>PRSLANAPIMILNGPNLNLLGQRQPEIYGSDTLADVEALCVK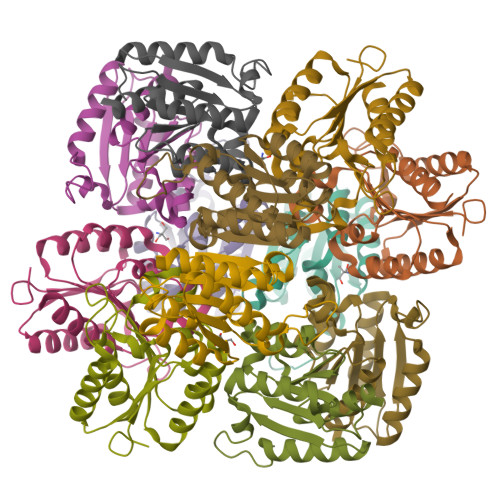AAAAHGGTVDFRQSNHEGELVDWIHEARLNHCGIVINPAAYSHTSVAILDALNTCDGLPVVEVHISNIHQREPFRHHSYVSQRADGVVAGCGVQGYVFGVERIAALAGAGSARA[12x]> QPHIIQLKNETTYENGQVTLVCDAEGEPIPEITWKRAVDGFTFTEGDKSLDGRIEVKGQHGSSSLHIKDVKLSDSGRYDCEAASRIGGHQKSMYLDIEYAPKFISNQTIYYSWEGNPINISCDVKSNPPASIHWRRDKLVLPAKNTTNLKTYSTGRKMILEIAPTSDNDFGRYNCTATNHIGTRFQEYILALADVPSSPYGVKIIELSQTTAKVSFNKPDSHGGVPIHHYQVDVKEVASE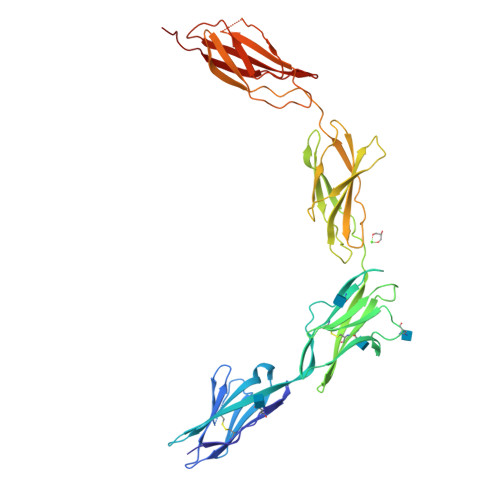IWKIVRSHGVQTMVVLNNLEPNTTYEIRVAAVNGKGQGDYSKIEIFQTLPVREPSPPSIHGQPSSGKSFKLSITKQDDGGAPILEYIVKYRSKDKEDQWLEKKVQGNKDHIILEHLQWTMGYEVQITAANRLGYSEPTVYEFSMPPKPN> ETGEEPPRFIKEPKDQIGVSGGVASFVCQATGDPKPRVTWNKKGKKVNSQRFETIEFDESAGAVLRIQPLRTPRDENVYECVAQNSVGEITVHAKLTVLREDQLPSGFPNIDMGPQLKVVERTRTATMLCAASGNPDPEITWFKDFLPVDPSASNGRIKQLRSGALQIESSEETDQGKYEC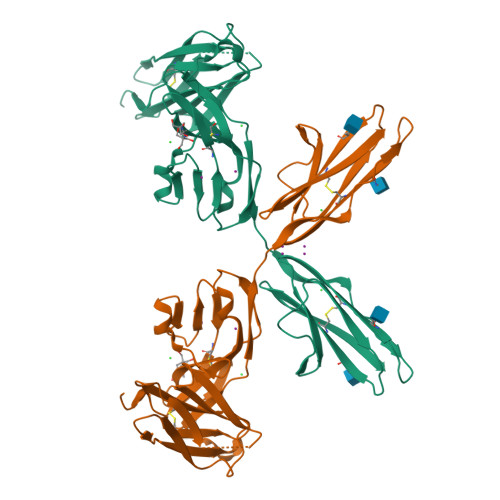VATNSAGVRYSSPANLYVRVQNVAPRFSILPMSHEIMPGGNVNITCVAVGSPMPYVKWMQGAEDLTPEDDMPVGRNVLELTDVKDSANYTCVAMSSLGVIEAVAQITVKSLPKAGTKHHHHHH>[6x]GSHMASNKYKRIFLVVMDSVGIGEAPDAEQFGDLGSDTIGHIAEHMNGLQMPNMVKLGLGNIREMKGISKVEK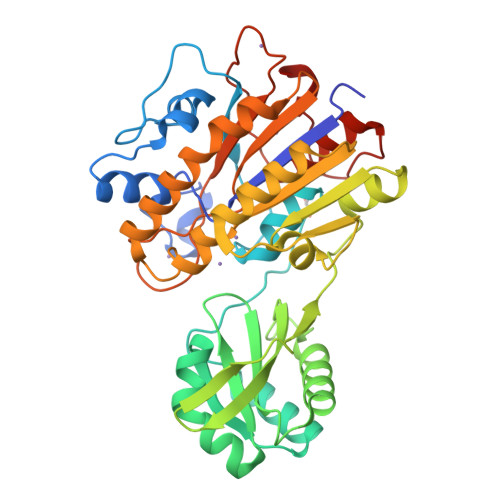PLGYYTKMQEKSTGKDEMTGHWEIMGLYIDTPFQVFPEGFPKELLDELEEKTGRKIIGNKPASGTEILDELGQEQMETGSLIVYTSADSVLQIAAHEEVVPLDELYKICKIARELTLDEKYMVGRVIARPFVGEPGNFTRTPNRHDYALKPFGRTVMNELKDSDYDVIAIGKISDIYDGEGVTESLRTKSNMDGMDKLVDTLNMDFTGLSFLNLVDFDALFGHRRDPQGYGEALQEYDARLPEVFAKLKEDDLLLITADHGNDPIHPGTDHTREYVPLLAYSPSMKEGGQELPLRQTFADIGATVAENFGVKMPEYGTSFLNELKK>[2x]AGPTAVPLGTAGNYAILASTAVSTVPQSAITGAVGISPAAGTFLTGFSLTMSGTGTFSTSTQVTGQLTAADYGTPTPSILTTAIGDMGTAYTNGATRSGPDFLEIYTGALGGTTLLPGLYKWTSSVGASADFTISGTSTDTWIFQIDGTLGLAAGKKITLAGGAQAKNIIWVVAGAVSIEAGAQFEGVILAKTAVTLKTGSSLNGRILAQTSVALQSATVVQK

Antifreeze proteins (AFPs) inhibit ice growth by adsorbing onto specific ice planes. To probe the molecular mechanisms responsible for AFP activity, we here characterized the antifreeze activity and crystal structure of TisAFP7 from the snow mold fungus Typhula ishikariensis. TisAFP7 exhibited intermediate activity, with the ability to bind the basal plane, compared with a hyperactive isoform TisAFP8 and a moderately active isoform TisAFP6. The structure is dominated by a right-handed β-helical domain, a typical DUF3494 structure.

The crystal structure of TisAFP7 was determined at 1.54 Å resolution by a molecular replacement method. The crystal belongs to the orthorhombic space group P212121, with unit cell parameters of a = 57.12 Å, b = 62.99 Å, and c = 101.21 Å, with two molecules in an asymmetrical unit. The final structure was refined with R factor of 0.195 and Free R factor of 0.229, and was composed of 446 (223 × 2) residues and 746 solvent molecules. The refined TisAFP7 structure exhibited the root-mean–squared deviation (RMSD) of 0.37 Å and 0.34 Å from Cα atoms of TisAFP6 and TisAFP8, respectively, reflecting high sequence identities shared by the isoforms. Analysis of the TisAFP7 crystal structure revealed a bound-water network arranged in a zigzag pattern on the surface of the protein’s ice-binding site (IBS). Among the approximately 54 waters molecules on IBS, six water molecules were aligned in a small trough formed by the inward-facing hydrophobic residues (Val22, Val213, Val195, Val177, Leu150, and Val126) at the β-sheet region of IBS. The interval between water molecules 3 and 6 was 14.51 Å, which closely matched that between the water molecules in a prism ice plane (4.6 Å and 14.7 Å). To survey the bound water structure in the IBS loop region in detail, we next compared the structure of TisAFP7 with those of TisAFP6 and TisAFP8. In all these isoforms, 12 water molecules in corresponding positions formed a zigzag-pattern network with branches, shown by red spheres in Fig. 6a. The average distance between the comprising water molecules and the nearest carbon atom of the interior aromatic side chain was 3.4 Å, which implies that these water molecules were constrained to engage in hydrophobic interactions with the Phe43 side chain.> MEEPEEPADSGQSLVPVYIYSPEYVSMCDSLAKIPKRASMVHSLIEAYALHKQMRIVKPKVASMEEMATFHTDAYLQHLQKVSQEGDDDHPDSIEYGLGYDCPATEGIFDYAAAIGGATITAAQCLIDGMCKVAINWSGGWHHAKKDEASGFCYLNDAVLGILRLRRKFERILYVDLDLHHGDGVEDAFSFTSKVMTVSLHKFSPGFFPGTGDVSDVGLGKGRYYSVNVPIQDGIQDEKYYQICESVLKEVYQAFNPKAVVLQLGADTIAGDPMCSFNMTPVGIGKCLKYILQWQLATLILGGGGYN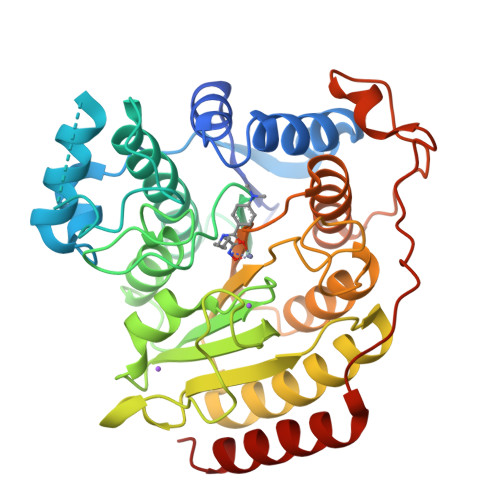LANTARCWTYLTGVILGKTLSSEIPDHEFFTAYGPDYVLEITPSCRPDRNEPHRIQQILNYIKGNLKHVV> MAAEEGVASAASAGGSWGTAAMGRVLPMLLVPVPAEAMGQLGSRAQLRTQPEALGSLTAAGSLQVLSLTPGSRGGGRCCLEGPFWHFLWEDSRNSSTPTEKPKLLALGENYELLIYEFNLKDGRCDATILYSCSREALQKLIDDQDISISLLSLRILSFHNNTSLLFINKCVILHIIFPERDAAIRVLNCFTLPLPAQAVDMIIDTQLCRGILFVLSSLGWIYIFDVVDGTYVAHVDLALHKEDMCNEQQQEPAKISSFTSLKVSQDLDVAVIVSSSNSAVALNLNLYFRQHPGHLLCERILEDLPIQGPKGVDEDDPVNSAYNMKLAKFSFQIDRSWKAQLSSLNETIKNSKLEVSCCAPWFQDILHLESPESGNHSTSVQSWAFIPQDIMHGQYNVLQKDHAKTSDPGRSWKIMHISEQEEPIELKCVSVTGFTALFTWEVERMGYTITLWDLETQGMQCFSLGTKCIPVDSSGDQQLCFVLTENGLSLILFGLTQEEFLNRLMIHGSASTVDTLCHLNGWGRCSIPIHALEAGIENRQLDTVNFFLKSKENLFNPSSKSSVSDQFDHLSSHLYLRNVEELIPALDLLCSAIRESYSEPQSKHFSEQLLNLTLSFLNNQIKELFIHTEELDEHLQKGVNILTSYINELRTFMIKFPWKLTDAIDEYDVHENVPKVKESNIWKKLSFEEVIASAILNNKIPEAQTFFRIDSHSAQKLEELIGIGLNLVFDNLKKNNIKEASELLKNMGFDVKGQLLKICFYTTNKNIRDFLVEILKEKNYFSEKEKRTIDFVHQVEKLYLGHFQENMQIQSFPRYWIKEQDFFKHKSVLDSFLKYDCKDEFNKQDHRIVLNWALWWDQLTQESILLPRISPEEYKSYSPEALWRYLTARHDWLNIILWIGEFQTQHSYASLQQNKWPLLTVDVINQNTSCNNYMRNEILDKLARNGVFLASELEDFECFLLRLSRIGGVIQDTLPVQNYKTKEGWDFHSQFILYCLEHSLQHLLYVYLDCYKLSPENCPFLEKKELHEAHPWFEFLVQCRQVASNLTDPKLIFQASLANAQILIPTNQASVSSMLLEGHTLLALATTMYSPGGVSQVVQNEENENCLKKVDPQLLKMALTPYPKLKTALFPQCTPPSVLPSDITIYHLIQSLSPFDPSRLFGWQSANTLAIGDAWSHLPHFSSPDLVNKYAIVERLNFAYYLHNGRPSFAFGTFLVQELIKSKTPKQLIQQVGNEAYVIGLSSFHIPSIGAACVCFLELLGLDSLKLRVDMKVANIILSYKCRNEDAQYSFIRESVAEKLSKLADGEKTTTEELLVLLEEGTWNSIQQQEIKRLSSESSSQWALVVQFCRLHNMKLSISYLRECAKANDW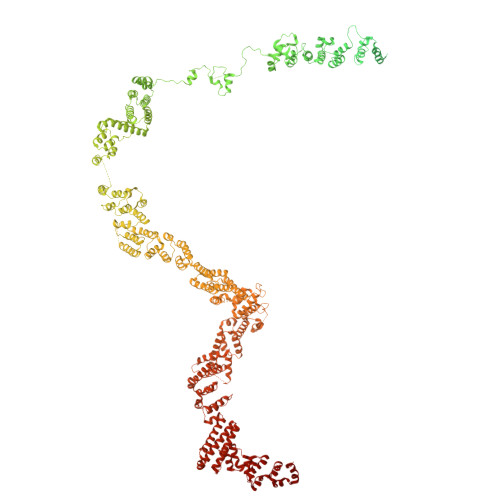LQFIIHSQLHNYHPAEVKSLIQYFSPVIQDHLRLAFENLPSVPTSKMDSDQVCNKCPQELQGSKQEMTDLFEILLQCSEEPDSWHWLLVEAVKQQAPILSVLASCLQGASAISCLCVWIITSVEDNVATEAMGHIQDSTEDHTWNLEDLSVIWRTLLTRQKSKTLIRGFQLFFKDSPLLLVMEMYELCMFFRNYKEAEAKLLEFQKSLETLNTAATKVHPVIPAMWLEDQVCFLLKLMLQQCKTQYELGKLLQLFVEREHLFSDGPDVKKLCILCQILKDTSIAINHTIITSYSIENLQHECRSILERLQTDGQFALARRVAELAELPVDNLVIKEITQEMQTLKHIEQWSLKQARIDFWKKCHENFKKNSISSKAASSFFSTQAHVACEHPTGWSSMEERHLLLTLAGHWLAQEDVVPLDKLEELEKQIWLCRITQHTLGRNQEETEPRFSRQISTSGELSFDSLASEFSFSKLAALNTSKYLELNSLPSKETCENRLDWKEQESLNFLIGRLLDDGCVHEASRVCRYFHFYNPDVALVLHCRALASGEASMEDLHPEIHALLQSAELLEEEAPDIPLRRVHSTSSLDSQKFVTVPSSNEVVTNLEVLTSKCLHGKNYCRQVLCLYDLAKELGCSYTDVAAQDGEAMLRKILASQQPDRCKRAQAFISTQGLKPDTVAELVAEEVTRELLTSSQGTGHKQMFNPTEESQTFLQLTTLCQDRTLVGMKLLDKISSVPHGELSCTTELLILAHHCFTLTCHMEGIIRVLQAAHMLTDNHLAPSEEYGLVVRLLTGIGRYNEMTYIFDLLHKKHYFEVLMRKKLDPSGTLKTALLDYIKRCRPGDSEKHNMIALCFSMCREIGENHEAAARIQLKLIESQPWEDSLKDGHQLKQLLLKALTLMLDAAESYAKDSCVRQAQHCQRLTKLITLQIHFLNTGQNTMLINLGRHKLMDCILALPRFYQASIVAEAYDFVPDWAEILYQQVILKGDFNYLEEFKQQRLLKSSIFEEISKKYKQHQPTDMVMENLKKLLTYCEDVYLYYKLAYEHKFYEIVNVLLKDPQTGCCLKDMLAG>[11x]MHHHHHHENLYFQGMSGTEEAILGGRDSHPAAGGGSVLCFGQCQYTAEEYQAIQKALRQRLGPEYISSRMAGGGQKVCYIEGHRVINLANEMFGYNGWAHSITQQNVDFVDLNNGKFYVGVCAFVRVQLKDGSYHEDVGYGVSEGLKSKALSLE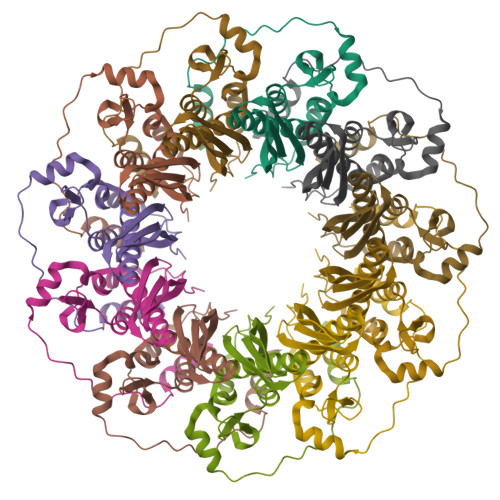KARKEAVTDGLKRALRSFGNALGNCILDKDYLRSLNKLPRQLPLEVDLTKAKRQDLEPSVEEARYNSCRPNMALGHPQLQQVTSPSRPSHAVIPADQDCSSRSLSSSAVESEATHQRKLRQKQLQQQFRERMEKQQVRVSTPSAEKSEAAPPAPPVTHSTPVTVSEPLLEKDFLAGVTQELIKTLEDNSEKWAVTPDAGDGVVKPSSRADPAQTSDTLALNNQMVTQNRTPHSVCHQKPQAKSGSWDLQTYSADQRTTGNWESHRKSQDMKKRKYDPS> MALRGTVTDFSGFDGRADAEVLRKAMKGLGTDEDSILNLLTARSNAQRQQIAEEFKTLFGRDLVNDMKSELTGKFEKLIVALMKPSRLYDAYELKHALKGAGTDEKVLTEIIASRTPEELRAIKQAYEEEYGSNLEDDVVGDTSGYYQRMLVVLLQANRDPDCAIDDAQVELDAQALFQAGELKWGTDEEKFITILGTRSVSHLRRVFDKYMTISGFQIEETIDRETSGNLENLLLAVVKSIRS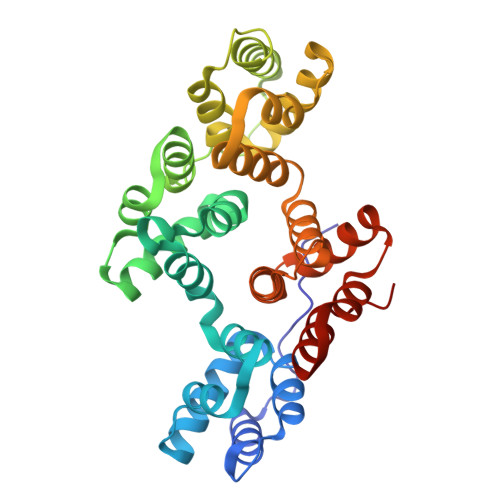IPAYLAETLYYAMKGAGTDDHTLIRVIVSRSEIDLFNIRKEFRKNFATSLYSMIKGDTSGDYKKALLLLSGGED>GAMDMSWTDERVSTLKKLWLDGLSASQIAKQLGGVTRN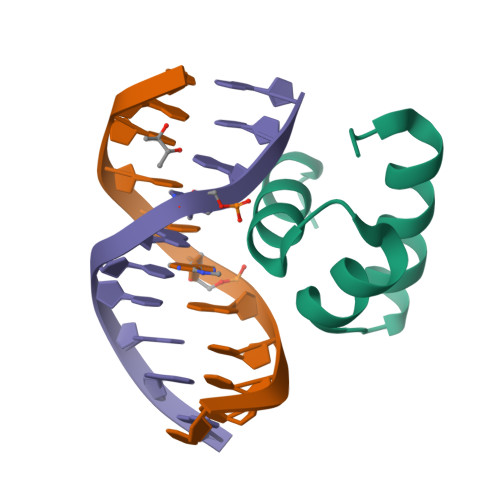AVIGKVHRLGL[3x]[FeFe]-hydrogenases represent one of natures’ most effective classes of redox enzymes catalyzing the reversible reduction of protons to dihydrogen (H2) at turnover frequencies of up to 9000 s-11–3. With their low catalytic over-potential, [FeFe]-hydrogenases represent excellent models for a regenerative and likewise economically feasible H2 production. Their active center (“H-cluster”) can be structured into a standard [4Fe-4S]-cluster ([4Fe]H) and a diiron site ([2Fe]H). Theoretical studies suggest that the most probable PT pathway comprises of strictly conserved residues E282, S319, E279, and C299 (from surface to H-cluster, numbering corresponds to CpI), including two protein-bound water molecules (Wat826, Wat1120 4XDC19, chain B) located between E279 and C29915,16,20. In this study, site-directed mutagenesis (SDM) is used to investigate the PT pathway of two [FeFe]-hydrogenases, namely CpI and HydA1, which represent the largest (M3) and smallest (M1) type of monomeric [FeFe]-hydrogenases, respectively.

Corresponding to earlier crystal structure data, for all CpI variants a space group of P1 21 1 was observed with two copies in the asymmetric unit cell (chain A and B). In case of C299DCpI, the carboxyl group of the side chain establishes H-bonds (2.7 Å) with the amine group of [2Fe]H and the “conserved” water molecule Wat708 (corresponding to Wat826 in chain B of 4XDC19). Unsurprisingly, protein samples of C169DHydA1 and C299DCpI both retain a rather high level of H2 release activity (30–80%). The favorable position of the acidic asparagine side chain in the structure of C299DCpI effectively connects adt-NH of the [2Fe]H moiety with the conserved water molecule Wat708 in the otherwise intact PT pathway, rendering this variant significantly active. This comparatively high level of absolute activity and the fact that both corresponding variants, C169DHydA1 and C299DCpI, exhibit significant shifts in their pH-dependent activity optimum to the acidic range might explain why this type of variant refuses to accumulate Hhyd even at pH 4, while instead effectively continuing the turnover process as evident according to the comparatively dominant infrared bands for the reduced states Hred and Hsred (1890 and 1882 cm−1 for C169D) recorded at pH 4. With the exception of S189AHydA1/S319ACpI, these variants retain a higher level of H2-release activity, which explains why in these cases Hhyd cannot be trapped at pH 8; just as wild-type enzyme, these variants populate Hhyd when titrated to significantly lower pH values. Interestingly, variant C169D and the corresponding variant of CpI (C299D) seem to be incapable of accumulating Hhyd under any of the conditions applied here. The strongest impacts were achieved when replacing E279CpI for A or Q, or C299CpI for A or S, resulting in activities <1%.

>MKTIIINGVQFNTDEDTTILKFARDNNIDISALCFLNNCNNDINKCEICTVEVEGTGLVTACDTLIEDGMIINTNSDAVNEKIKSRISQLLDIHEFKCGPCNRRENCEFLKLVIKYKARASKPFLPKDKTEYVDERSKSLTVDRTKCLLCGRCVNACGKNTETYAMKFLNKNGKTIIGAEDEKCFDDTNCLLCGQCIIACPVAALSEKSHMDRVKNALNAPEKHVIVAMAPSVRASIGELFNMGFGVDVTGKIYTALRQLGFDKIFDINFGADMTIMEEATELVQRIENNGPFPMFTSDCPGWVRQAENYYPELLNNLSSAKSPQQIFGTASKTYYPSISGLDPKNVFTVTVMPCTSKKFEADRPQMEKDGLRDIDAVITTRELAKMIKDAKIPFAKLEDSEADPAMGEYSGAGAIFGATGGVMEAALRSAKDFAENAELEDIEYKQVRGLNGIKEAEVEINNNKYNVAVINGASNLFKFMKSGMINEKQYHFIEVMACHGGCVNGGGQPHVNPKDLEKVDIKKVRASVLYNQDEHLSKRKSHENTALVKMYQNYFGKPGEGRAHEILHFKYKKSAWSHPQFEK[2x]>[4x]GASGSMVEKNGAKKTSLRELPKISDRVSFIYVEHAKINRVDSAITVLDSRGTVRIPAAMIGVLLLGPGTDISHRAVELIGDTGTSMVWVGERGVRQYAHGRSLAHSTKFLEKQAKLVSNSRLRLAVARKMYQMRFPDEDVSAMTMQQLRGREGARVRRVYRLQSEKYQVSWTKREYNPDDFEGG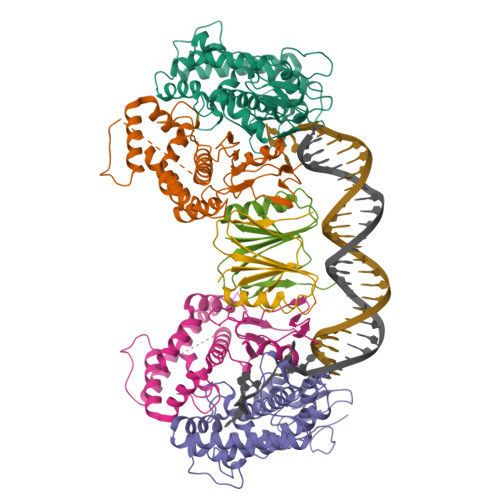DIVNQALSAANVALYGLVHSIVIALGASPGLGFVHTGHDLSFIYDIADLYKAELTIPLAFEIAANFTEIDDIGKIARQKVRDSFVDGKLIVRIVQDIQYLFDLDDDEELLVDTLSLWDDKDMLVKHGVSYKEEL;>MPFTVVTLKSVPPSLRGDLTKWMQEIAIGVYVGNFNSRIREKLWNRIQANVGEGEATISYYYRNEIGYQFDMINSQKSVVDFDGIPLVLIPNSKTSSENYPKLGYSNAAKSRKIKRYSSYRG[2x]> GPAMAKVETGTDVTSKVTVEIGSIEGHNNTNKVEPHAGQRAVLKYKLKFENGLHQGDYFDFTLSNNVNTHGVSTARKVPEIKNGSVVMATGEVLEGGKIRYTFTNDIEDKVDVTAELEINLFIDPKTVQTNGNQTITSTLNEEQTSKELDVKYKDG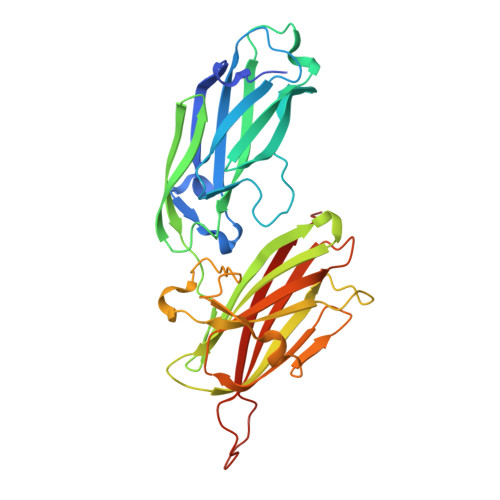IGNYYANLNGSIETFNKANNRFSHVAFIKPNNGKTTSVTVTGTLMKGSNQNGNQPKVRIFEYLGNNEDIAKSVYANTTDTSKFKEVTSNMSGNLNLQNNGSYSLNIENLDKTYVVHYDGEYLNGTDEVDFRTQMVGHPEQLYKYYYDRGYTLTWDNGLVLYSNKA> MAITPEQIAVEYPIPTYRFVVSVGDEQIPFNNVSGLDV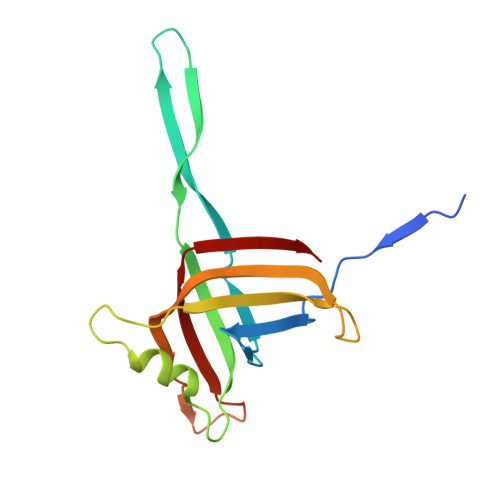HYDVIEYKDGIGNYYKMPGQRQSINITLRKGVFPGDTKLFDWINSIQLNQVEKKDIAISLTNEAGTEILMTWNVANAFPTSFTSPSFDATSNEIAVQEIALTADRVTIQAA The neural cell adhesion molecule (NCAM) is the prototype and founding member of the immunoglobulin (Ig) superfamily cell adhesion molecules (CAMs). NCAM is present on the cell surface of neurons, astrocytes and oligodendrocytes, where it mediates homophilic and heterophilic cell adhesion. NCAM is involved in neuronal migration, axon growth and guidance, as well as in synaptic plasticity associated with learning and memory. We conclude that the NCAM–FGFR1 interaction at the cell surface may be transient or stabilised by avidity effects resulting from receptor clustering and that conformational changes within NCAM may have a profound role in FGFR1 activation.

Our structure is of the shortest isoform (linker sequence TQPVREPSAP), whereas the underlined arginine residue is replaced by QG, HSPPPQG or even longer sequences in other variants. We do not think that the dimer observed in our crystals is physiologically relevant, as dimer interface residues are only poorly conserved and NCAM dimers were never observed in electron microscopy studies. In agreement with our earlier prediction, the FRM and FGL loops are indeed located in close proximity on the same face of the wild-type NCAM molecule. Intriguingly, the corresponding loop regions are in close proximity in the acutely bent conformation observed in crystals of the wild-type protein, suggesting that they are part of a larger FGFR1 binding site extending over the domain junction. The neuroglian tandem, which has an extensive domain interface that incorporates a bound sodium ion, adopts a conformation that is intermediate between the two conformations we report for the NCAM tandem. Thus, a similar bend in the FN3 linker(s) may be a general feature of other animal CAMs containing FN3 domains in their membrane-proximal region.

>APLAQADTPSSPSIDQVEPYSSTAQVQFDEPEATGGVPILKYKAEWRAVGEEVWHSKWYDAKEASMEGIVTIVGLKPETTYAVRLAALNGKGLGEISAASEFKTQPVREPSAPKLEGQMGEDGNSIKVNLIKQDDGGSPIRHYLVRYRALSSEWKPEIRLPSGSDHVMLKSLDWNAEYEVYVVAENQQGKSKAAHFVFRTAAAHHHHHH[2x]> MPLVYTPAVRGGANPASGSYLLDPQYVNSGVDILQATYGYNING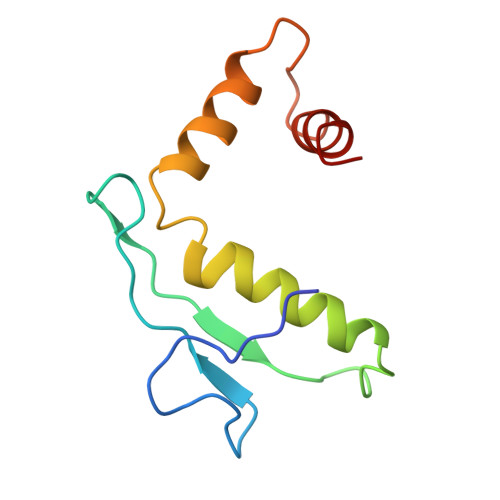TANADQLLQRDAILAILEYALKDTAFVNAIQAVAAGSGVTTPASFVSACVTKLTA[{2-[(guanine-9-yl)methyl]propane-1,3-diyl}bis(oxymethylene)]bis(phosphonic 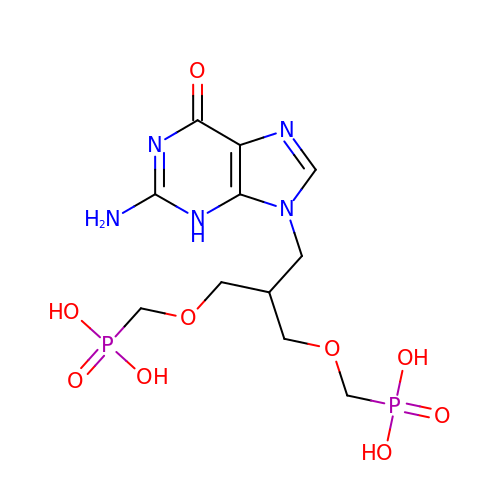acid)  | C11 H19 N5 O9 P2 | VGXYLSOVNUSSKA-UHFFFAOYSA-N>GPLGSQFLVYKNIIKDYIQSRLFNEGLLDGPYRCDIKDVKTKKVSERLKEVGNELEGKFKDSFSNMCERLTITDTTAYPTFVGVVNELFSTGINWGRIVAFIVFSSRLAIHFKRNGMPEYVKSVYGWVARYMHTKLSTWIEANRSWDGFLDHFD[2x];>PSSPTSEIGRHLAQLGDSYSVRFQNE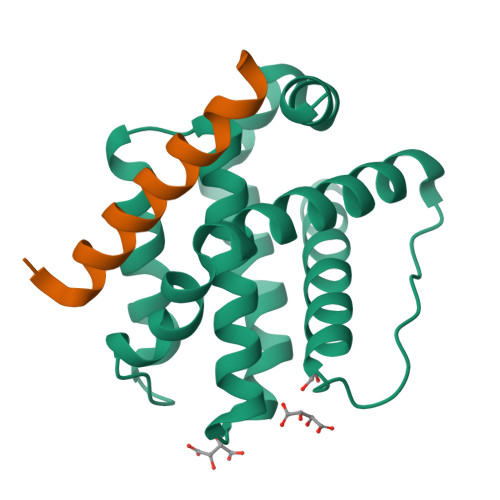[2x]> MLDGPYQPTTFTPPNDYWILINSNTNGVVYESTNNSDFWTAVVAI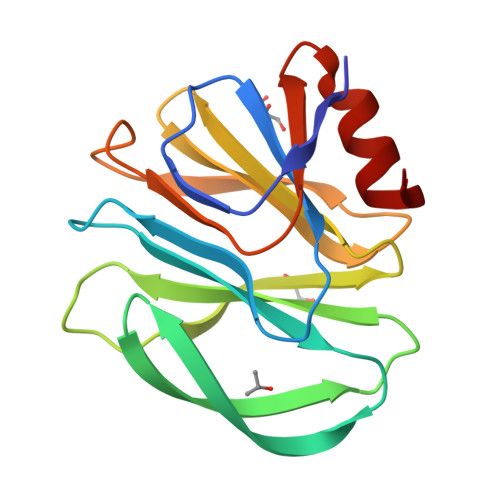EPHVNPVDRQYTIFGESKQFNVSNDSNKWKFLEMFRSSSQNEFYNRRTLTSDTRLVGILKYGGRVWTFHGETPRATTDSSSTANLNNISITIHSEFYIIPRSQESKCNEYINNGL> GQYKDNIRHGVCWIYYPDGGSLVGEVNEDGEMTGEKIAYVYPDERTALYGKFIDGEMIEGKLATLMSTEEGRPHFELMPGNSVYHFDKSTSSCISTNALLPDPYESERVYVAESLISSAGEGLFSKVAVGPNTVMSFYNGVRITHQEVDSRDWALNGNTLSLDEETVIDVPEPYNHVSKYCASLGHKANHSFTPNCIYDMFVHPRFGPIKCIRTLRAVEADEELTVAYGYDH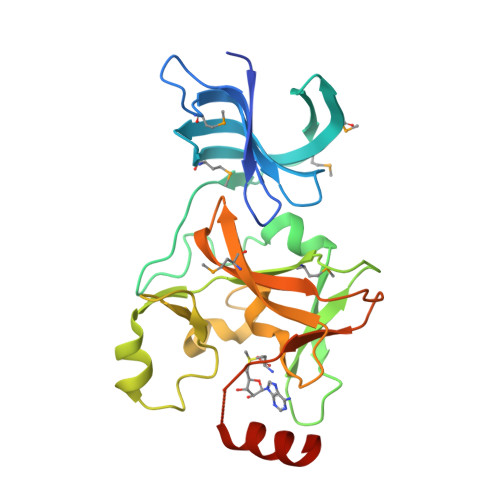SPPGKSGPEAPEWYQVELKAFQATQQK>[2x]MSEGRRGLGRGLSALLGEVDAAPAQAPGEQLGGSREAPIEILQRNPDQPRRTFREEDLEDLSNSIREKGVLQPILVRPSPDTAGEYQIVAGERRWRAAQRAGLKTVPIMVRELDDLAVLEIGIIENVQRADLNVLEEALSYKVLMEKFERTQENIAQTIGKSRSHVANTMRLLALPDEVQSYLVSGELTAGHARAIAAAADPVALAKQIIEGGLSVRETEALARKAPNLSAGKSKGGRPPRVKDKLAAALEHHHHHH

In most bacterial species, faithful chromosome segregation is mediated by the tripartite ParA-ParB-parS system. ParB, a CTPase and DNA-binding protein, nucleates on parS before spreading to adjacent non-specific DNA to form a higher-order nucleoprotein complex. The ParB-DNA nucleoprotein complex stimulates the ATPase activity of ParA, driving the movement of the parS locus (and subsequently, the whole chromosome) to the opposite pole of the cell. ParB spreads by sliding along the DNA, in a manner that depends on the binding of a co-factor, cytidine triphosphate (CTP) (Balaguer F de et al., 2021; Jalal et al., 2020c; Osorio-Valeriano et al., 2019; Soh et al., 2019).

Next, to gain insight into the spreading state of ParB, we solved a 2.7 Å resolution structure of C. crescentus ParB∆CTD in complex with CTPɣS. Hence, we modeled CTP, instead of CTPɣS, into the electron density. The asymmetric unit contains two copies of ParB∆CTD, each with a CTPɣS molecule and a coordinated Mg2+ ion bound at the NTD. In contrast to the open conformation of the ParB∆CTD-parS structure, nucleotide-bound NTDs from opposite subunits self-dimerize (with an interface area of 2111 Å2, as determined by PISA; Krissinel, 2015), thus adopting a closed conformation. Each CTPɣS molecule is sandwiched between helices α1, α2, α3 from one subunit and helix α3′ from the opposite subunit. Ten amino acids form hydrogen-bonding contacts with three phosphate groups of CTPɣS, either directly or via the coordinated Mg2+ ion. Four amino acids at helix α1 and the α1–β2 intervening loop provide hydrogen-bonding interactions to the cytosine ring, hence are termed the C-motif (C for cytosine motif). The C-motif forms a snug fit to the pyrimidine moiety, thus is incompatible with larger purine moieties such as those from ATP or GTP. However, in the spreading state, as represented by the ParB∆CTD-CTPɣS structure, α3 swings outwards by 101o to pack itself with α4′ from the opposing subunit. By overlaying the CTPɣS-bound structure onto the parS DNA complex, it is clear that the DBDs in the spreading state clash severely with DNA, hence are no longer compatible with parS DNA binding.6-ethyl-5-[3-(5-methoxybiphenyl-3-yl)prop-1-yn-1-yl]pyrimidine-2,4-diamine | C22 H22 N4 O | 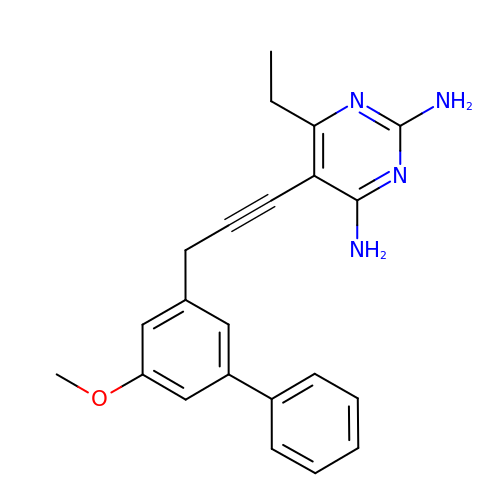QKLZHVMWTSBUFL-UHFFFAOYSA-N>MKTDKLDMNAKRQLYSLIGYASLRLHYVTVKKPTAVDPNSIVECRVGDGTVLGTGVGRNIKIAGIRA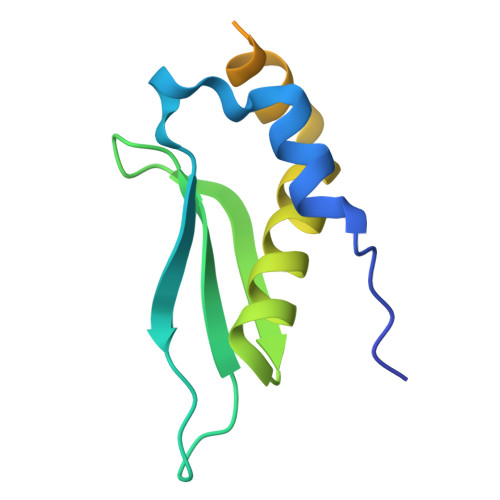AENALRDKKMLDFYAKQRAAIPRSESVLKDPSQKNKKRKFSDTSHHHHHH[2x]>MIQSQINRNIRLDLADAILLSKAKKDLSFAEIADGTGLAEAFVTAALLGQQALPADAARLVGAKLDLDEDSILLLQMIPLRGCIDDRIPTDPTMFRFYEMLQVYGTTLKALVHEKFGDGIISAINFKLDVKKVADPEGGERAVITLDGKYLPTKP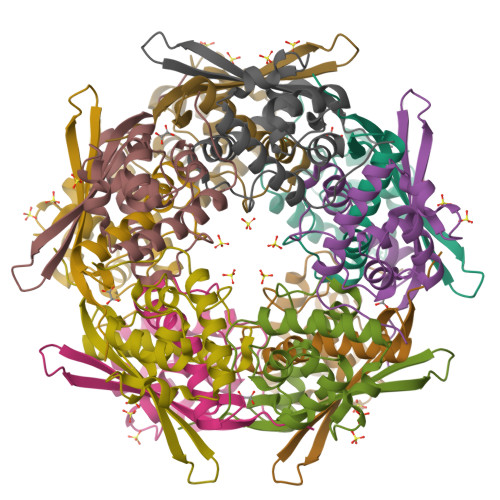F[10x]In this study, we co-crystalized ELIC with the general anesthetic isoflurane, which is known to inhibit mammalian neuronal and muscle nAChRs3132 and GLIC33. The crystal structures of ELIC-isoflurane were determined with resolutions of 3.0 Å and 3.4 Å in the absence and presence of agonists, corresponding to the presumed resting and desensitized states of ELIC, respectively. As a homolog to eukaryotic pLGICs, ELIC shares similar pharmacological profiles of eukaryotic cation-conducting pLGICs with respect to modulation by general anesthetics. Thus, isoflurane inhibition via a direct pore-binding mechanism is likely accomplished jointly by stabilizing the closed channel conformation and blocking the open channel.

For ELIC crystallized with isoflurane but without an agonist (presumed in the resting state), the FO-FC omit electron density map shows strong electron densities for double isoflurane occupancies inside the pore near residues T237(6′) and A244(13′). Nearly equal electron densities observed at the two sites suggest that isoflurane has similar binding affinities to both sites. Isoflurane at the 6′ position can form hydrogen bonds with the hydroxyl group of T237 in addition to hydrophobic contacts with L240 at the 9′ position, while isoflurane binding at the 13′ position is dominated by hydrophobic interactions with the side chain of L240. Over the course of the MD simulations of the resting ELIC, isoflurane remained near the same two sites (6′ and 13′) as revealed in the crystal structure. Isoflurane movement perpendicular to the channel axis was largely confined within 2 Å of the pore radius in two replicated simulations, indicating stable binding in the closed pore. The RMSF decreased in the closed ELIC bound stably with isoflurane compared to the RMSF of the apo ELIC. An open pore-blocking mechanism, however, cannot completely describe the isoflurane inhibition of ELIC since isoflurane also occupies the pore of ELIC in the resting state. Furthermore, isoflurane binding to the resting pore stabilizes a closed channel conformation. Although T237(6′) and A244(13′) have different side-chain volumes (T = 120 Å3 vs. A = 90 Å3), the tilting of the TM2 helix makes the pore radii at the 6′ and 13′ positions nearly the same (∼3 Å). The binding site at 6′ consists of side chains of all five T237(6′) and two L240(9′) residues that form a favorable amphipathic environment to stabilize isoflurane binding through amphipathic interactions.

>APADNAADARPVDVSVSIFINKIYGVNTLEQTYKVDGYIVAQWTGKPRKTPGDKPLIVENTQIERWINNGLWVPALEFINVVGSPDTGNKRLMLFPDGRVIYNARFLGSFSNDMDFRLFPFDRQQFVLELEPFSYNNQQLRFSDIQVYTENIDNEEIDEWWIRGKASTHISDIRYDHLSSVQPNQNEFSRITVRIDAVRNPSYYLWSFILPLGLIIAASWSVFWLESFSERLQTSFTLMLTVVAYAFYTSNILPRLPYTTVIDQMIIAGYGSIFAAILLIIFAHHRQANGVEDDLLIQRCRLAFPLGFLAIGCVLVIRGITL[10x]>RGQRGEVEQMKSCLRVLSQPMPPTAGEAEQAA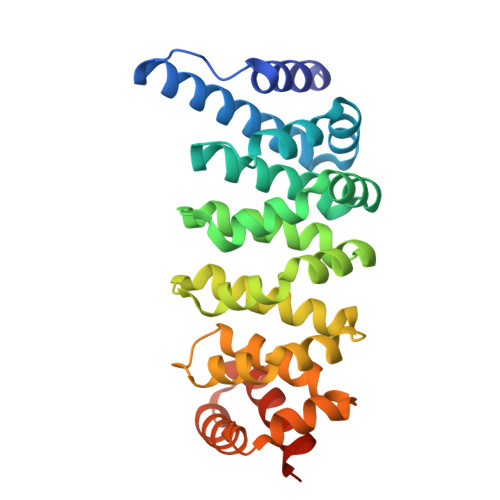DQQEREGALELLADLCENMDNAADFCQLSGMHLLVGRYLEAGAAGLRWRAAQLIGTCSQNVAAIQEQVLGLGALRKLLRLLDRDACDTVRVKALFAISCLVREQEAGLLQFLRLDGFSVLMRAMQQQVQKLKVKSAFLLQNLLVGHPEHKGTLCSMGMVQQLVALVRTEHSPFHEHVLGALCSLVTDFPQGVRECREPELGLEELLRHRCQLLQQHEEYQEELEFCEKLLQTCFSSPADDSMDR[4x]Flexible filamentous viruses are ubiquitous plant pathogens that have an enormous impact in agriculture. Their infective particles are non-enveloped and flexible rod-shaped virions and contain several hundreds of copies of a coat protein (CP) arranged in a helical fashion protecting a ssRNA of positive polarity, or (+)ssRNA. Pepino mosaic virus (PepMV) is another potexvirus which has emerged recently, progressing from endemic to epidemic in tomato crops causing severe economic losses worldwide. PepMV is transmitted by mechanical contact and virions contain a (+)ssRNA of about 6.4 kb. The PepMV CP is strictly required for cell-to-cell movement of the virus.

We present the cryoEM structure of PepMV virions at 3.9 Å of resolution. The cryoEM map reveals a left-handed helix with a diameter of 130 Å and an inner narrow channel of 13 Å, and the structure shows a pitch of 34.6 Å and 8.7 CP copies per turn. The PepMV CP structure thus generated has three major regions: the core; an N-terminal flexible arm; and a C-terminal extension. The first 20 amino acids in the N-terminal side are not included in the atomic model because the region projects outwards, and its density vanishes due to high flexibility. Each CP binds five ribonucleotides, so that the entire genome of PepMV would require 1290 copies of PepMV CP spanning 510 nm (3.95 Å of axial rise/subunit), which agrees with the 509 nm length originally reported for the virus. In order to explore the protein–ssRNA interactions, we modeled a polyU and included a set of four PepMV CP monomers in a molecular dynamics flexible fitting (MDFF) simulation. The results show that the RNA resides in a continuous groove with a high electropositive potential constructed by CPs from consecutive turns of the helix. Three polar-charged residues, R124, D163, and K196 might establish H-bonding contacts with this RNA base. The N-terminal arm from the Ni subunit interacts with a hydrophobic groove of the Ni-1 subunit and establishes the main side-by-side contact in the helical arrangement. Thus, the C-terminal extensions are responsible for the axial interactions that support helix formation.

> MPDTTPVAATSSAPPTAKDAGAKAPSDFSNPNTAPSLSDLKKVKYVSTVTSVATPAEIEALGKIFTAMGLAANETGPAMWDLARAYADVQSSKSAQLIGATPSNPALSRRALAAQFDRINITPRQFCMYFAKVVWNILLDSNIPPANWAKLGYQEDTKFAAFDFFDGVTNPASLQPADGLIRQPNEKELAAHSVAKYGALARQKISTGNYITTLGEVTRGHMGGANTMYAIDAPPEL Tryptophan-2,3-dioxygenase (TDO2) and indoleamine-2,3-dioxygenase (IDO1) are structurally distinct heme enzymes that catalyze the conversion of L-tryptophan to N-formyl-kynurenine, and play important roles in metabolism, inflammation, and tumor immune surveillance. Tryptophan-2,3-dioxygenase (TDO2) and indoleamine-2,3-dioxygenase 1 (IDO1) catalyze the same reaction: the conversion of L-tryptophan (Trp) to N-formyl-kynurenine (NFK). Both enzymes evolved to bind heme for substrate binding and catalysis but are structurally distinct: IDO1 is monomeric, while TDO2 is tetrameric with two independent TDO2 molecules contributing to each of its four active sites. The enzymes can adopt an inactive, heme-free (apo) state or an active, heme-containing (holo) state, with the balance between them varying dynamically according to biological conditions. While apo-TDO2 is catalytically inactive, the term “apo-TDO2 inhibitor” is used to describe compounds that bind to apo-TDO2, compete with heme binding and thus prevent the formation of enzymatically active holo-TDO2.

Two steps were essential for successful co-crystallization of apo-TDO. First, apo-TDO2 was expressed using an E. coli strain that is unable to synthesize heme. Second, the exosite binder AMT was added to apo-TDO2 because of its stabilizing effect as observed in DSF experiments. An exosite that binds both the substrate Trp and its α-methyl analog AMT has been identified previously in holo-TDO224. AMT led to an improved apo-TDO2 melting curve quality and was therefore included in all apo-TDO2 inhibitor DSF measurements. In the presence of AMT, apo-TDO2 could be crystallized both alone and in complex with the inhibitor Cpd-2.

>GLIYGNYLHLEKVLNAQELQSETKGNKIHDEHLFIITHQAYELWFKQILWELDSVREIFQNGHVRDERNMLKVVSRMHRVSVILKLLVQQFSILETMTALDFNDFREYLSPASGFQSLQFRLLENKIGVLQNMRVPYNRRHYRDNFKGEENELLLKSEQEKTLLELVEAWLERTPGLEPHGFNFWGKLEKNITRGLEEEFIRIQAKEESEEKEEQVAEFQKQKEVLLSLFDEKRHEHLLSKGERRLSYRALQGALMIYFYREEPRFQVPFQLLTSLMDIDSLMTKWRYNHVCMVHRMLGSKAGTGGSSGYHYLRSTVSDRYKVFVDLFNLSTYLIPRHWIPKMNPTIHKFLEHHH[4x]>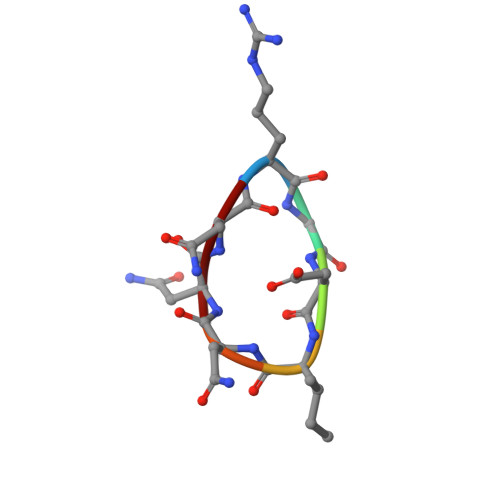 RGDINNN>[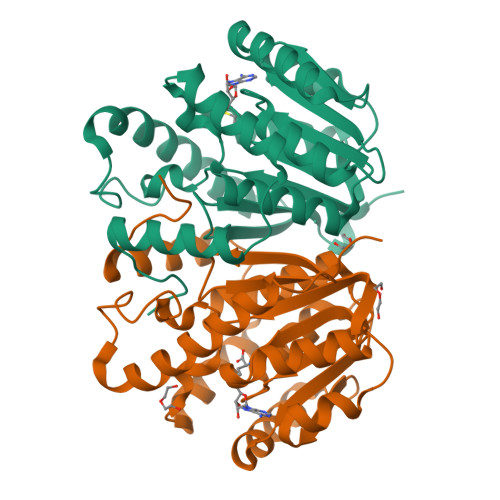4x]MLGSILPFNEETADRVSAYCEKNSHGIPDALVEHWEWTRTRFPDADKMSSRLQGSWMIFTARDRKPKRILEIGCYSGYSALAWYEGTRDTKAEIVTLEYSPKMIAASREAFKKYGVGDRVKLIEGPAENTLKTLEGEFDLIFVDANKDGYAGYVKTILDQGLLSANGIILCDNVFARGLTIGPDCAPWLNDHVRPYWNGCGQALDKFSAGLMEDPRIDVLLLPVFDGVTQIRWKDGAQRA>GSHMKNVSGSVKLWVDTTQVPYYKKIVANFNKKYPDVKVKVTQSPNGSANAKTDVGKDPAKAADVFEVANDQLGSMAEAGYINPLSPDATKAVKNNNVAVASEGVTWKGKMFAYPFAEQAQTIYYNKSKLTADDVKTWDGLTAKGVLATDFTNAYNFYPVFLSAGTQLYGKTGETVKGTDVNSAKGEQAMAWFAQQKSNKGVMQTSNALNQLKSGKAAAILDGPWNSANIKKILGKNFAVAPYPTIKLDGKDVQMQAFLGIET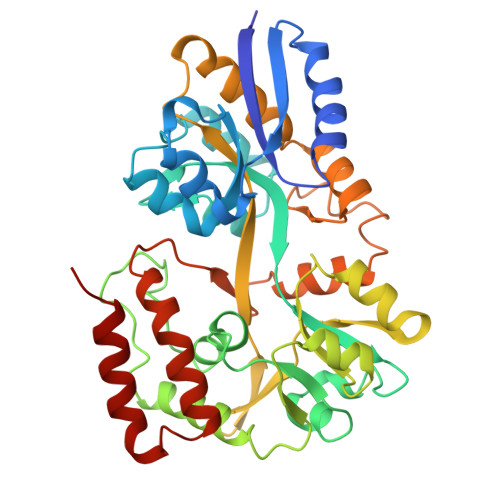FAVNSHASGSNQKAAATLASFITNKESQLIVYDHSGQIPVDKTAQKSSKVASDPVAGAVMTMAKPGNSTLMPKMPQMATFWNDAAPLINGAYTGSIPASQYSTKLDTFVKNISKAN[8x]>GSGAWKASVDPLGVVGSGADVYLYFPVAGNENLISRIIENHESKADIKKIVDRTTAVYGAFFARSKEFRLFGSGSYPYAFTNLIFSRSDGWASTKTEHGITYYESEHTDVSIPAPHFSCVIFGSSKRERMSKMLSRLVNPDRPQLPPRFEKECTSEGTSQTVALYI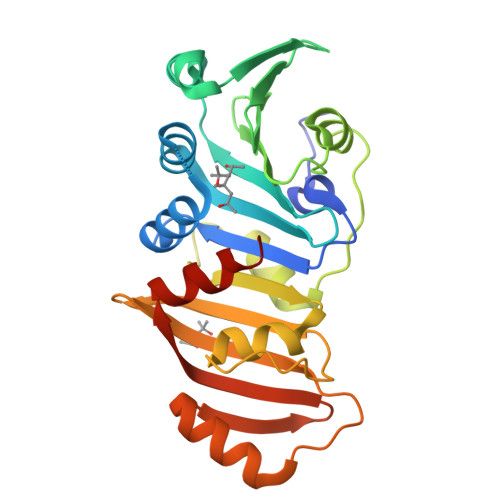KNGGHFITKLLNFPQLNLPLGAMELYLTARRNEYLYTLSLQLGNAKINFPIQFLISRVLNAHIHVEGDRLIIEDGTISAERLASVISSLYSKKGSS[2x]>MGQLLQTLTGHSSSVTGVAFSPDGQTIASASDDKTVKLWNRNGQLLQTLTGHSSSVTGVAFSPDGQTIASASDDKTVKLWNRNGQLLQTLTGHSSSVTGVAFSPDGQTIASASDDKTVKLWNRNGQLLQTLTGHSSSVTGVAFSPDGQTIASASDDKTVKLWNRNGQLLQTLTGH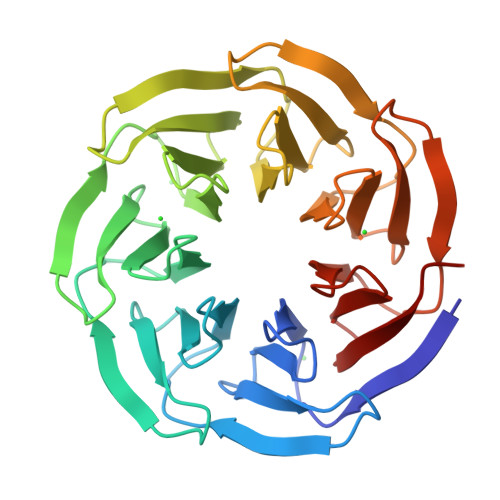SSSVTGVAFSPDGQTIASASDDKTVKLWNRNGQLLQTLTGHSSSVTGVAFSPDGQTIASASDDKTVKLWNRNGQLLQTLTGHSSSVTGVAFSPDGQTIASASDDKTVKLWNRN[2x]>[4x]MATGNPEGKKRPPEEQRL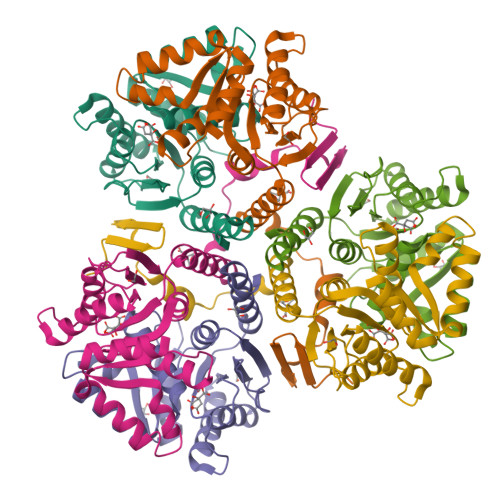GPVLRRRGQVQESTTDQRLLDERAPTDWVHTDPWRVLRIQSEFIEGFGTLAELPPAISVFGSARTPADSPEYDAGVRLGRGLVEAGFAVITGGGPGAMEAANKGALEAKGTSVGLGIELPFEQGLNPYVDIGLNFRYFFVRKMMFVKYAQGFVVLPGGLGTLDELFEALTLVQTQKVTRFPIVLFGSEYWGGLVDWLRGTLVAQGKAAEKDLMLFHVTDDVDEAVALVSKEAGRLEHHHHHH>[4x]MSGESGQPEAGPSHAGLDWPNPERNRAGVPGGVIRRAGSQGPRSWIQKVLEQIMDSPRQCVTPSEVVPVTVLAVQRYLLEDEPRDTVPKPPLYCYD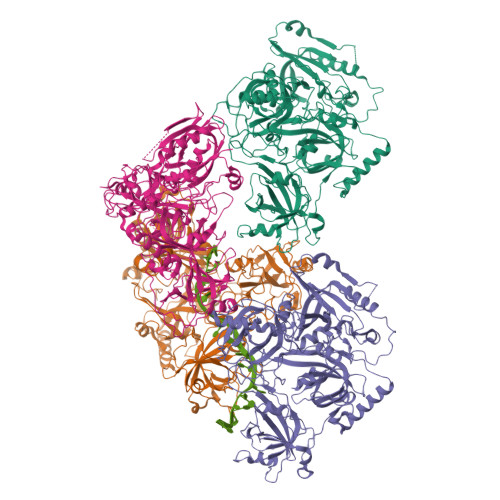VTISDGVYQEKCYLDPSLNSLVYQNILKVGIQMRISRVSCLYNEKRIGQGILCIDNVHCGETSDSISLETPFRNRAHQEKPERPLRGGKSHYLALWNNEDPYGDIWLTDKQPEEHNFSDTKIISLSHLEMTWTNRRNFPALLVRILHKSKLRYYGKPDKKMIEPYQTFLEVADSSGTVSVIMWNALCPEWYKSLRVGLVLLLQDYSVKKSYPFRIQPVPVDPQIKLISTMEICLNLRDPPTNIIIIPEKQVKPEWRLPKLNHRFTTRSELDDMPENCICDVIGLLVFVGRVQRSKKKENREDFWSYRWIHIADGTSEQPFIVELFSTSQPEIFENIYPMAYFVCTQLKVVRNDNQVPKLLYLTTTNESGVFITGHRGQPYTYDAKVKNFIQWIRTKSDSGEQKNMVIGGYYPYPPVPETFSKYSSSIKVESLLTAISEVRKEIEDLQYREQKRIAIQGIITAIKYIPHSSATESASASETLRNANRPSTSQAARVEIQERNGKRHQDDEPVNSQYFQTTSTNLSLSNKIRILQGPHANPVAVPQPGASVQTKGIKPGMPSIFNRRANINANLQGKARKTISDRWESQLWREKKFGLIDHLHYSRVYPESIPRKFMFEHRKFLSDQYNSQPAKYVPPEGRPPKLDDFKSARSLGHFEVTILGLNHEIAIDVAFLPMYCPEDIRTSQIDTLLTSMNYSCAYPQDTTGNDRLPGPRAVAGDIIKAATELDRVHIVGILDICNLGNNKVEVYLHKIYSPENTS(3~{R})-1-(2-chlorophenyl)pyrrolidine-3-carboxylic acid | C11 H12 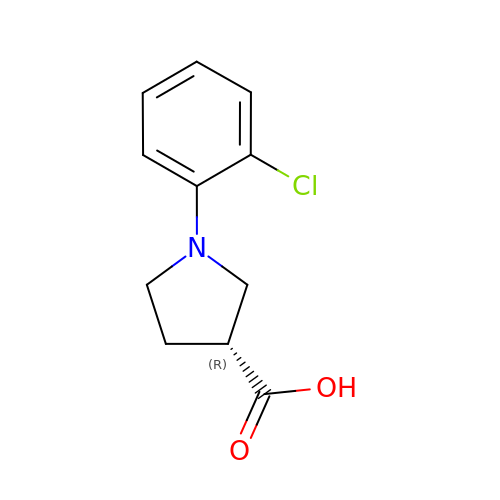Cl N O2 | FPGYADRKFPWWLU-MRVPVSSYSA-N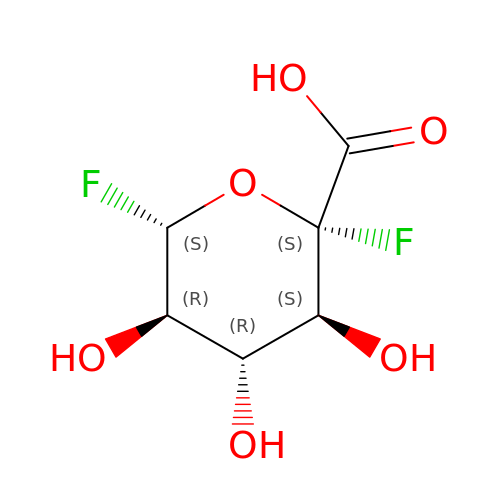5-fluoro-alpha-L-idopyranosyluronic acid fluoride | C6 H8 F2 O6 | NQKZMBDISJYOPD-ORELYVPDSA-N> 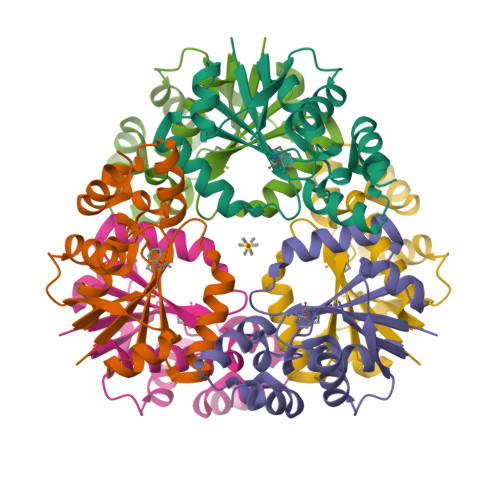GSMTGAVCPGSFDPVTLGHVDIFERAAAQFDEVVVAILVNPAKTGMFDLDERIAMVKESTTHLPNLRVQVGHGLVVDFVRSCGMTAIVKGLRTGTDFEYELQMAQMNKHIAGVDTFFVATAPRYSFVSSSLAKEVAMLGGDVSELLPEPVNRRLRDRLNTERT>GPGETQNLNSGWTDTAHGSGIIPMRTDLELDFSLPSSASYTYRRQLQNPANEQEKIPFHLQISKQVIHAEIQHLGHWMDGTFNLKTAFHCYGSCEKYAYPWQTAGCFIEKDYEYESGWGCNPPDCPGVGTGCTACGVYLDKLKSVGKAFKIVSLRYTRKACIQLGTEQTCKSVDSNDCLVTTSVKVCLIGTVSKFQPSDTLLFLGPLEQGGLIFKQWCTTTCQFGDPGDIMSTPVGMKCPELNGSFRKKCAFATTPVCQFDGNTLSGYKRMIATKDSFQSFNVTEPHISASSLEWIDPDSSLRDHINVIVGRDLSFQDLSETPCQVDLATTSIDGAWGSGVGFNLVCSVSLTECSTFLTSIKACDSAMCYGSTTANLLRGQNTVHIVGKGGHSGSKFMCCHDTKCSSTGLVAAAPHLDRVTGYNQADSDKIFDDGAPECGISCWFTKSGEGTETSQVAPA[2x];>[2x]ETGELKIECPHTIGLGQGLVIGSVELPPVPLTQVESLKLESSCNFDLHTSTSSQQPFTKWTWEMKSDLAENTQASSTSFQTKSSEINLRGLCLVPPLVIETAARTRKTIACFDLSCNQTACQPTVFLIGPIQTCITTKSCLLGLGDQRIQVNYEKTYCVSGQLVEGVCFNPVHTMALSQPSHTYDIVTVMVRCFLIAKKVSTGDSMKLEKSFETLVQKTSCTGNGFQGYYICLVGSSSEPLYIPTLDDYRSAEVLSRMAFAPHGEDHDVEKNAISAMRIIGKVTGKAPSTESSDTIQGVAFSGNPL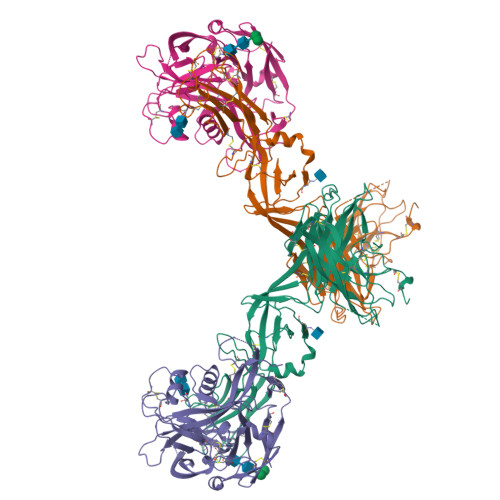YTSTGVLTAKDDPVYIWAPGIIMEGNHSVCDKKTLPLTWTGFIPLPGEIEKTGTKHHHHHH> VVGGTEAQRNSWPSQISLQYRSGSSWAHTCGGTLIRQNWVMTAAHCVDRELTFR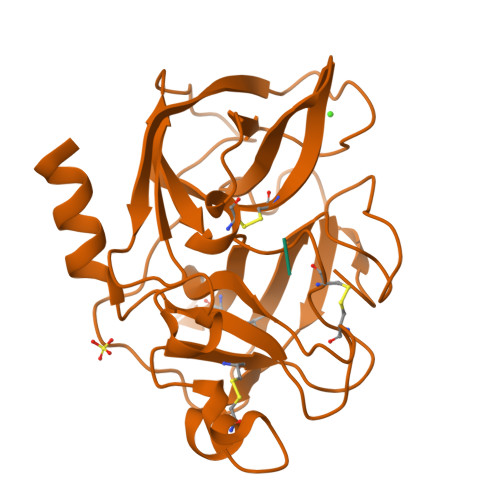VVVGEHNLNQNNGTEQYVGVQKIVVHPYWNTDDVAAGYDIALLRLAQSVTLNSYVQLGVLPRAGTILANNSPCYITGWGLTRTNGQLAQTLQQAYLPTVDYAICSSSSYWGSTVKNSMVCAGGDGVRSGCQGDSGGPLHCLVNGQYAVHGVTSFVSRLGCNVTRKPTVFTRVSAYISWINNVIASN;> YPFVEPIK> GHMSMQGPRTRPRKPIRAGEVLFAVGGWASGDAISSVERYDPQTNEWRMVASMSKRRCGVGVSVLDDLLYAVGGHDGSSYLNSVERYDPKTNQWSSDVAPTSTARTSVGVAVLGGFLYAVGGQDGVSALNIVERYDPKKNKWTRVASMSTRRLGVAVAVLGGFLYAVGGSDGT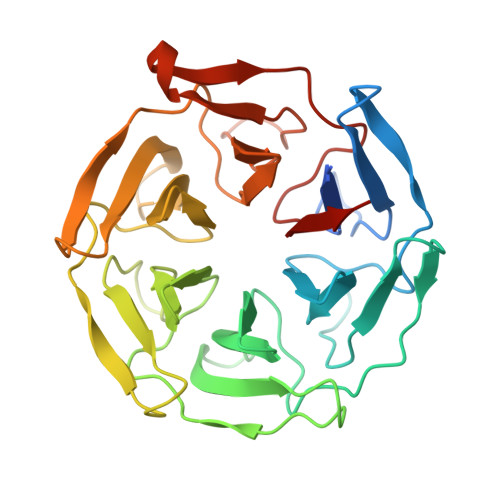SPLNTVERYNPQENRWHTIAPMGTRRKHLGCAVYQDMIYAVGGRDDTTELSSAERYNPRTNQWSPVVAMTSRRSGVGLAVVNGQLMAVGGFDGTTYLKTIEVFDPDANTWRLYGGMNYRRLGGGVGVIKMTHAE>SMADRNLRDLLAPWVPDAPSRALREMTLDSRVAAAGDLFVAVVGHQADGRRYIPQAIAQGVAAIIAEAKDEATDGEIREMHGVPVIYLSQLNERLSALAGRFYHEPSDNLRLVGVTGTNGKTTTTQLLAQWSQLLGEISAVMGTVGNGLLGKVIPTENTTGSAVDVQHELAGLVDQGATFCAMEVSSHGLVQHRVAALKFAASVFTNLSRDHLDYHGDMEHYEAAKWLLYSEHHCGQAIINADDEVGRRWLAKLPDAVAVSMEDHINPNSHGRWLKATEVNYH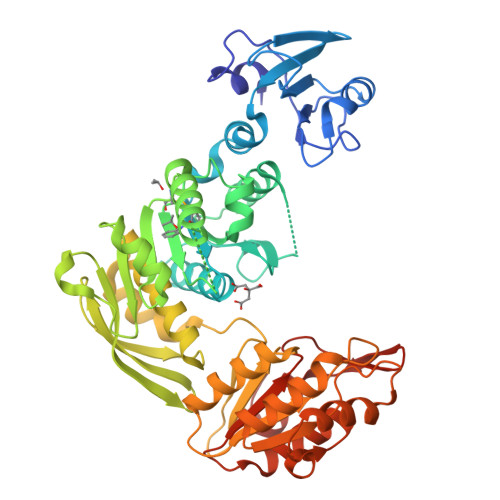DSGATIRFSSSWGDGEIESHLMGAFNVSNLLLALATLLALGYPLADLLKTAARLQPVSGRMEVFTAPGKPTVVVDYAHTPDALEKALQAARLHCAGKLWCVFGCGGDRDKGKRPLMGAIAEEFADVAVVTDDNPRTEEPRAIINDILAGMLDAGHAKVMEGRAEAVTSAVMQAKENDVVLVAGKGHEDYQIVGNQRLDYSDRVTVARLLGVIA[2x]>HGAVTSYNIAGKDYPGYSGFAPTGQDVIQWQWPDYNPVLSASDPKLRCNGGTGAALYAEAAPGDTITATWAQWTHSQGPILVWMYKCPGDFSSCDGSGAGWFKIDEAGFHGDGTTVFLDTETPSGWDIAKLVGGNKSWSSKIPDGLAPGNYLVRHELIALHQANNPQFYPECAQIKVTGSGTAEPAASYKAAIPGYCQQSDPNISFNINDHSLPQEYKIPGPPVFKGTASAK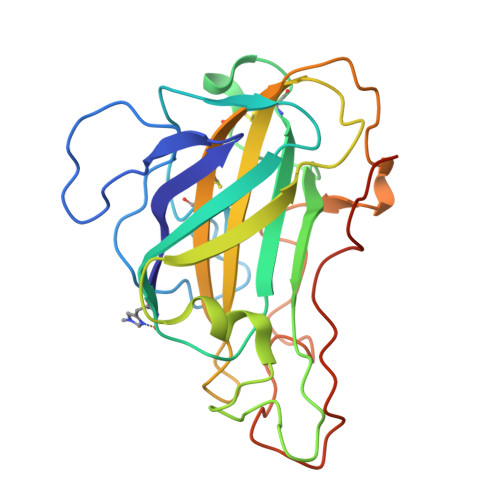ARAFQA[6x]Here, we show that a novel Mn-dependent peroxidase is an important factor in tardigrade anhydrobiosis. We crystallized the putative globular domain that lacked the N-terminus 62 amino acids of g12777 protein (g12777-Δ62) and solved the crystal structures as two forms containing Mn2+ or Zn2+ ions at 2.30 Å and 1.60 Å resolutions, respectively. The functional assays conducted here suggest that g12777 is a manganese-dependent peroxidase, independent of other components of the cell.

The Mn2+-bound g12777 crystals prepared by soaking method (50 mM Mn2+) using Zn2+-bound crystals indicated that the Zn2+ ion in the Zn-1 site was replaced with Mn2+. Additionally, an Mn2+ ion was found to be bound at a new binding site (Mn-2), whereas the Zn2+ in Zn-2–5 disappeared. A part of the β5–β6 loop (residues 163–168) around the Mn2+-binding site was disordered in the Mn2+-bound crystal, suggesting its flexible nature. In the Mn2+-binding site located at the negatively charged patch comprising β1–β2 and β3–β4 loops, the side-chain oxygen atoms of Asp92, Asp98, and Asp131 and the main-chain carbonyl atom of Ala96 and two water molecules coordinate with Mn2+ ion at distances of 2.2–2.9 Å. A considerable conformational difference was observed between Mn2+- and Zn2+-bound forms in terms of the metal-binding site, in which Asp92 and Asp98 were commonly involved in Mn2+ and Zn2+ binding. These aspartic acid residues were highly conserved within tardigrade orthologs, and the highly conserved CD-CD motif containing two Asp residues (D92 and D98) was used in the metal ion binding in both structures, suggesting the importance of these residues. The presence of a disulfide bond close to the Mn-1 binding site is suggestive of the utilization of the disulfide bond as an electron acceptor, which could categorize this protein as a new class of peroxidase. The recombinant β-sandwich domain of g12777 protein (g12777-Δ62) showed significant peroxidase activity when Mn2+ ions but not Zn2+ ions were present. The sample buffer used for this assay contains 0.1% BSA, and the manufacturer warrants the lack of non-specific protein catalysis by BSA up to 1 mg/ml with this kit. This reaction (H2O2 + CH3OH → HCHO + 2H2O) was carried out without the presence of hemes, thus suggesting that this protein is distinguished from most Mn peroxidases. Furthermore, we speculate that this affinity is related to the localization of this protein mainly in the Golgi apparatus since it has a strictly controlled high manganese concentration, suggesting the antioxidative stress functionality in the Golgi apparatus seems to be crucial for anhydrobiotic survival.

>[2x]GSHMGRFADFFRIETEIQRLDNPAGILANGKKCDFTGACDPVVTAFLDLESPLSPWPGSVAASKWKTIFEATDQNSPTIGRSVIRDMCGGSASNVNLRVLVNDADSLSSQDEIGKFSCLFQLDARDVAMDSLSAQWGPSTECTAEAQQGKIRLFARRRAFEIPSTSCRAPSSL Containing a tandem array of 2–30 repeats, pentatricopeptide repeat (PPR) proteins constitute one of the largest protein families in land plants. Each PPR repeat aligns to a single nucleotide of the RNA target in modular patterns, making these proteins suitable for the development of exciting new biotechnologies. Within each repeat, the combinations of two amino acids, known as the PPR code at two key positions (the 5th and the 35th) confer RNA specificity. A typical RNA-bound dPPR protein adopts a right-handed superhelical spiral structure, with its target ssRNA molecule sitting in the interior cavity and interacting with corresponding PPR repeats in a modular fashion.

On the basis of previous investigation, we used dPPR scaffolds with four different codes: ND, NS, SN and TD. After numerous unsuccessful trials, we finally succeeded in crystallizing each dPPR-U8N2 in complex with its respective target ssRNA (5′-UUUUNNUUUU-3′), in space group P212121. When dPPR-U8C2 was superimposed on dPPR-U10, dPPR-U8A2 and dPPR-U8G2, the root mean square deviations were 0.73, 0.99 and 1.00 Å over 348, 367 and 374 Cα atoms, respectively. As observed in all four complex structures, four types of dPPR repeats recognize their corresponding targets by forming hydrogen bonds with the Watson–Crick faces of the nucleotides, which explains why PPR proteins bind ssRNAs instead of double stranded ones. The amide group of the Asn5 side chain donates a hydrogen bond to the O2 atom of the corresponding pyrimidine, whereas the N3 atom of purine accepts a hydrogen bond from the hydroxyl group of the corresponding amino acid. We observed that water molecules between bases and PPR repeats mediate hydrogen bonds between the polar residues and the bases in the cases of uracil and cytosine recognition. Each water molecule between the base and corresponding PPR repeat forms two hydrogen bonds: one with the N3 atom of the pyrimidine and one with the carboxyl group of Asp35 or the hydroxyl group of Ser35. The N3 atom of uracil is a hydrogen bond donor, whereas the N3 atom of cytosine is a hydrogen bond acceptor. Interactions with the phosphate group of ssRNA, which are invariant for repeats 1 through 8, are mediated by salt bridges between Lys13 of repeat 1 and the 5′ phosphate group of U3, and between Lys13 of repeat 8 and the 5′ phosphate group of U10.

> ALLDETPLPPGSRLDVRAYTTVLHALSRAGRYERALELFAELRRQGVAPTVVTYNTLIDGLCKAGKLDEALKLFEEMVEKGIKPDVVTYNTLIDGLCKAGKLDEALKLFEEMVEKGIKPDVVTYNTLIDGLCKAGKLDEALKLFEEMVEKGIKPDVVTYNTLIDGLCKAGKLDEALKLFEEMVEKGIKPDVVTYNTLIDGLCKAGKLDEALKLFEEMVEKGIKPDVVTYNTLIDGLCKAGKLDEALKLFEEMVEKGIKPDVVTYNTLIDGLCKAGKLDEALKLFEEMVEKGIKPDVVTYNTLIDGLCKAGKLDEALKLFEEMVEKGIKPDVVTYNTLIDGLCKAGKLDEALKLFEEMVEKGIKPDVVTYNTLIDGLCKAGKLDEALKLFEEMVEKGIKPDELTYRRVVESYCRAKRFEEARGFLSEVSETDLDFDKKALEAYIEDAQFGRLEHHHHHHHH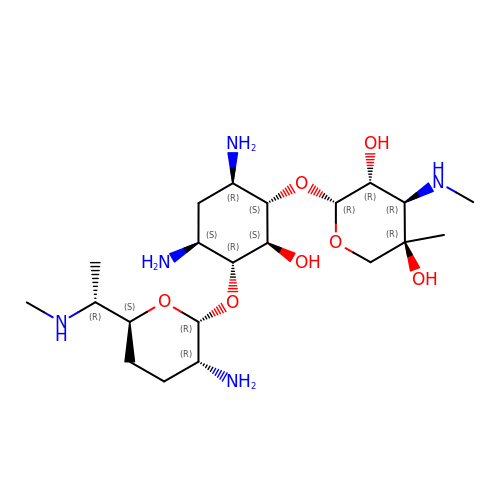gentamicin C1 | C21 H43 N5 O7 | CEAZRRDELHUEMR-CAMVTXANSA-N N-(5-cyclopropyl-1H-pyrazol-3-yl)-2-{(2R)-1-[(6-fluoropyridin-3-yl)carbonyl]pyrrolidin-2-yl}pyrrolo[2,1-f][1,2,4]triazin-4-amine | C22 H21 F N8 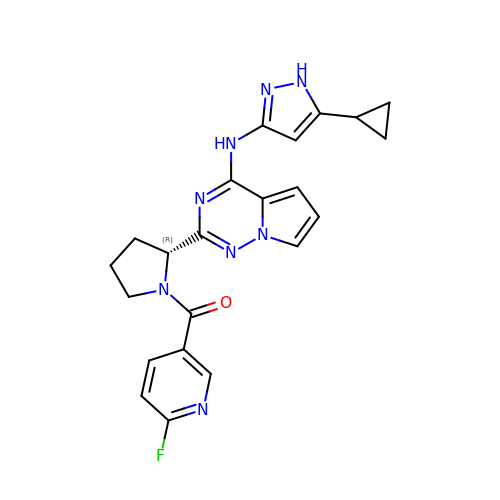O | XXGADWBTSMHVDF-MRXNPFEDSA-N> MNTPEHMTAVVQRYVAALNAGDLDGIVALFADDATVEGPVGSEPRSGTAAIREAYANSLKLPLAVELT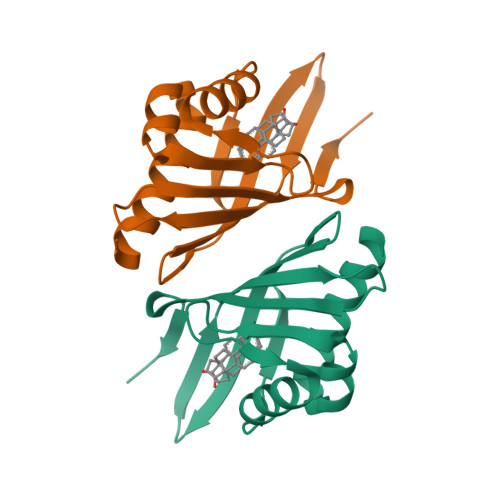QEVRAVANEAAFAFTVSFEYQGRKTVVAPIDHFRFNGAGKVVSMRALFGEKNIHAGA> SFDCGKPQVEPKKCPGRVVGGCVAHPHSWPWQVSLRTRFGMHFCGGTLISPEWVLTAAHCLEKSPRPSSYKVILGAHQEVNLEPHVQEIEVSRLFLEPTRKDIALLKLSSPAVITDKVIPACLPSPNYVVADRTECFITGWGETQGTFGAGLLKEAQLPVIENKVCNRYEFL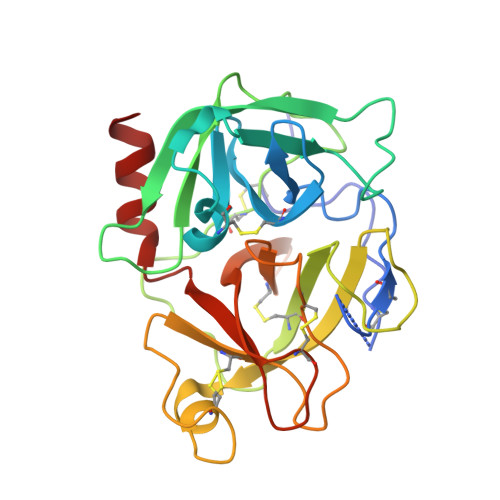NGRVQSTELCAGHLAGGTDSCQGDSGGPLVCFEKDKYILQGVTSWGLGCARPNKPGVYVRVSRFVTWIEGVMRNN>[4x]SMLTELIASNRRSAAIHAFVDTGLSTHFKDGIYVDISELSRKSGVNYAR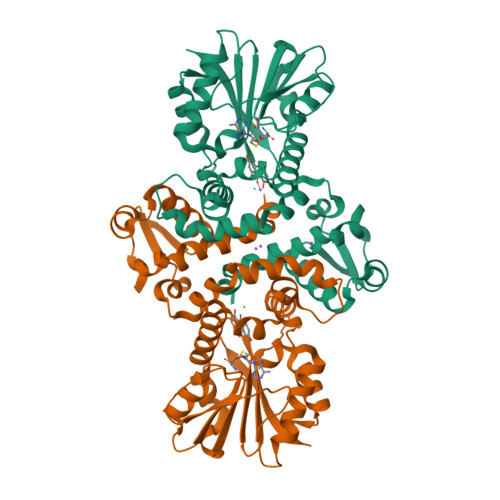FSRLCDFLVEMGVLVSNDNKFRLSDECHVFANPESFESFMIKLEICSHYSNAWLMYGKSLFEDDGKSAFEMAHGRPFFEYLDGNKFLKSNFDALMTRVSNLIVEKLLGIYDFNQHNRILDVGGGEGELLVRISEKVKGKHYAVLDRYSELPVSDNIDFINGNFLNSIPSGYDLYILKNVLHNWSDSDSILILENFRKAMDKNSSLLLINMVKEPEFSRSFDILMDVLFLGKERSFTEFEYLANQAGLVVQETKVIDQSYSPYSFIKLQIK> MKTQVAIIGAGPSGLLLGQLLHKAGIDNVILERQTPDYVLGKIRAGVLEQGMV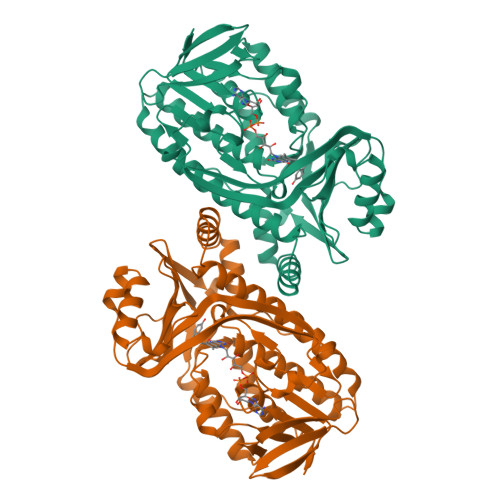DLLREAGVDRRMARDGLVHEGVEIAFAGQRRRIDLKRLSGGKTVTVYGQTEVTRDLMEAREASGATTVYQAAEVRLHDLQGERPYVTFERDGERLRLDCDYIAGCDGFHGISRQSIPAERLKVFERVYPFGWLGLLADTPPVSHELIYANHPRGFALCSQRSATRSRYYVQVPLTEKVEDWSDERFWTELKARLPAEVAEKLVTGPSLEKSIAPLRSFVVEPMQHGRLFLAGDAAHIVPPTGAKGLNLAASDVSTLYRLLLKAYREGRGELLERYSAICLRRIWKAERFSWWMTSVLHRFPDTDAFSQRIQQTELEYYLGSEAGLATIAENYVGLPYEEIE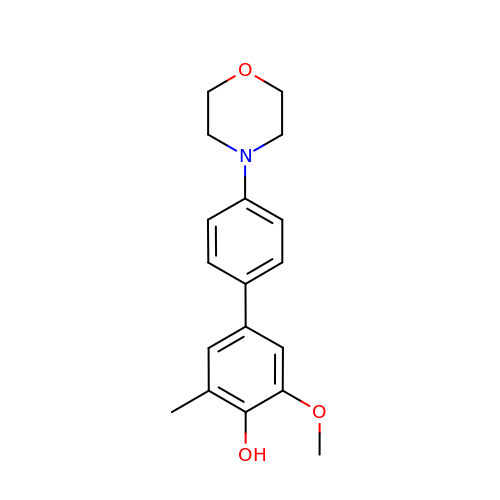3-methoxy-5-methyl-4'-(morpholin-4-yl)biphenyl-4-ol | C18 H21 N O3 | LUWYUXWJRQRONA-UHFFFAOYSA-N(5S,5aS,8aS,9S)-8-oxo-9-(3,4,5-trimethoxyphenyl)-5,5a,6,8,8a,9-hexahydrofuro[3',4':6,7]naphtho[2,3-d][1,3]dioxol-5-yl 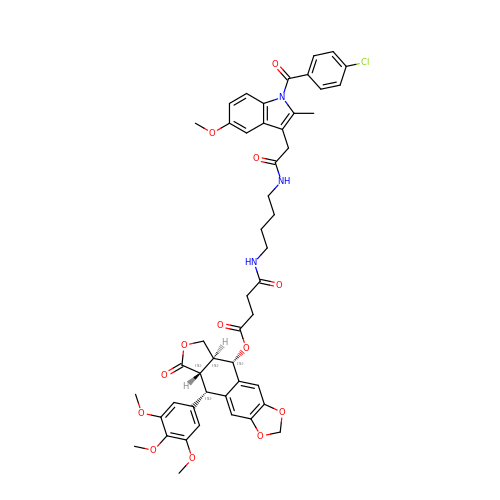4-{[4-({[1-(4-chlorobenzoyl)-5-methoxy-2-methyl-1H-indol-3-yl]acetyl}amino)butyl]amino}-4-oxobutanoate | C49 H50 Cl N3 O13 | VWODTBOQFNUCFF-XNSMRCHSSA-N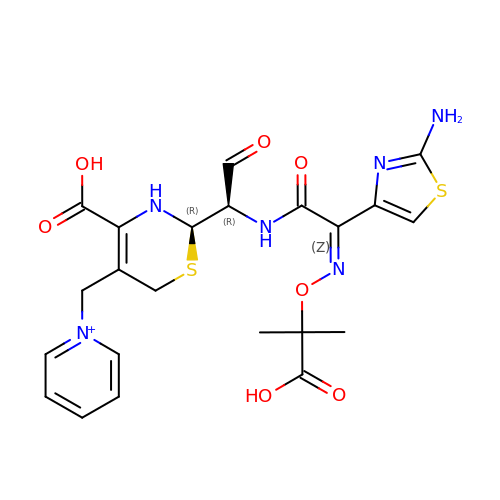1-({(2R)-2-[(1R)-1-{[(2Z)-2-(2-amino-1,3-thiazol-4-yl)-2-{[(2-carboxypropan-2-yl)oxy]imino}acetyl]amino}-2-oxoethyl]-4-carboxy-3,6-dihydro-2H-1,3-thiazin-5-yl}methyl)pyridinium | C22 H25 N6 O7 S2 | BJJNSFSVDFPVPL-QNLDICNMSA-O{[(1S,3R)-3-(5-methyl-2,4-dioxo-3,4-dihydropyrimidin-1(2H)-yl)cyclopentyl]oxy}propanedioic acid | C13 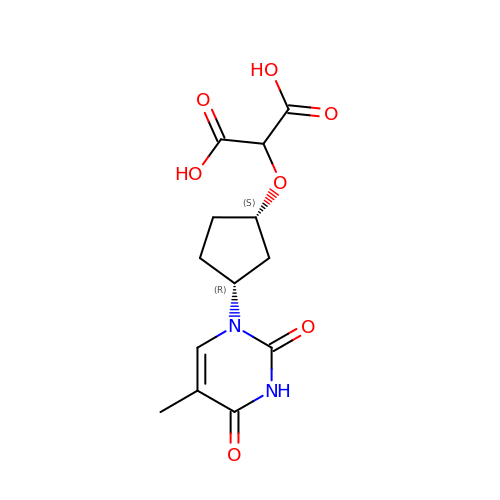H16 N2 O7 | LBUPGXBDONMGHG-SFYZADRCSA-N> HHHHHHMDKLKDTPFMVQVKLPNYKDYLLDNKQVVLTFKLVHHSKKITLIGDANKILQYKNYFQANGARSDIDFYLQP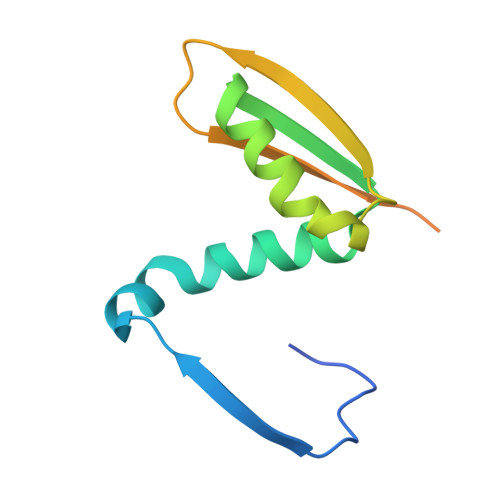TLNQKGVVMIASNYNDNPNSKEKPQTFDVLQGSQPMLGANT>MSQTLLVHGKDAQGIIKQVLSEVYDAVTSTMGPNGQLVMIKNGVSTKTTKDGVTVARSIRFADEAHELVNRVITEPATKTDEECGDGTTTTIMLTHALYHLFKDFPGFQHHRNIEDLVERVIQRLESMAIRVEVDDPRLYQVALTSSNQDEKLARLVSELYANNKGSYPDIELKEGVNFEDQIEQTTGRTIRMFYANPWFAKGHQGGVTELTGFTAFVIDRRIDKEDTQKLIDGVNHLVKTHKQHLALPILLIARSFEEAANSTLMQLNAAHPTLVEDGRPWLIPLSTPVGGAIGTSELQDIAVMLNAPMLSDVADLTKLDTHSINGQHGQLELGGNRSILKSTTPKDEDRIEQHARGIEELLEGFSLSDKFSVRARYNERRIRTLRGKLITISVGGETYSEVKERVDRYEDVVKAIRSALENGILPGGGVSLVKAVFGTIKEGLEDKDQSAEFAKRYINSGIANELMRLSTIQHKLLFKDTALYKENGSFHFNDDWLNTPTVMNLATGEIGTPEGLGIYDTAYASITALKGGLQTAKILATTKTLILGEKLSAVKVR[14x]

Our structural and functional analysis of the chaperonin ɸEL from the bacteriophage EL of P. aeruginosa revealed that the protein is ATPase active and functions in aggregation prevention of denatured proteins. ɸEL forms tetradecameric double ring complexes, which dissociate into a population of single rings in the presence of ATP and at physiological salt concentration. As anticipated, the ɸEL subunits displayed the typical three-domain architecture of chaperonins, composed of an equatorial domain (residues 2–130 and 425–552), an intermediate domain (residues 131–188 and 388–424), and an apical domain (residues 189–387). The domain structures of ɸEL differ from those of GroEL by numerous insertions and deletions, which alter the putative substrate-binding cleft and the contacts at the ring-ring interface. Our functional data rather suggests that the chaperone mechanism of ɸEL is encapsulation independent, and represents an evolutionary precursor of the more complex encapsulation mechanisms used by the group I and II chaperonins.

To mimic the conformational changes upon ATP-binding in solution, we also determined the cryo-EM structure of ɸEL in the presence of the slowly hydrolyzing ATP analog, ATPγS. Double-ring structures were again observed and symmetry-free 3D class averaging indicated nearly uniform rings. Applying D7 symmetry resulted in a refined cryo-EM density map at 5.8 Å resolution. The subunits assumed conformation I and were slightly tilted outward compared to ɸEL•ADP. Interestingly, we find a rotation at the ring-ring interface of 2.9° with a vertical displacement of 2.9 Å. This re-orientation would break the contacts between Asn465 and Glu466 with Asn465* and Arg469*/Gly462*, respectively. Moreover, the symmetrical van-der-Waals contact at the Lys486 residues can no longer form. Thus, binding of ATPγS weakens the ring-ring interface and this effect may be more pronounced in the presence of ATP, consistent with the finding of mainly single-rings in solution.> MGSSHHHHHSSGENLYFQGHMGKYTKKFNEVRSTDRPLVGGKCASLGEMVQAGLPVPDGFAVTIDAYEDFRDDSDLRAELRSLVFGVDPDSSKSLQDAHDQAVALVLGRNLPAAIEDEIREAYLTLSRETARRRGTGDTDRIPVAVRSSSVDEDGDAASFAGQQETYLWVVGADDVIAKVRECWASLYTPQAIAYRAGMSETDAAEASKISVAVQLMADADVAGVMFTVSPRTGDRSVIAINASWGLGQSVVSGEVTPDEYWLSKIGPTLTSSRIASKEHEYVPAPDGTGVIFREVEQARREVSCLSDSELMQLAEIGLRV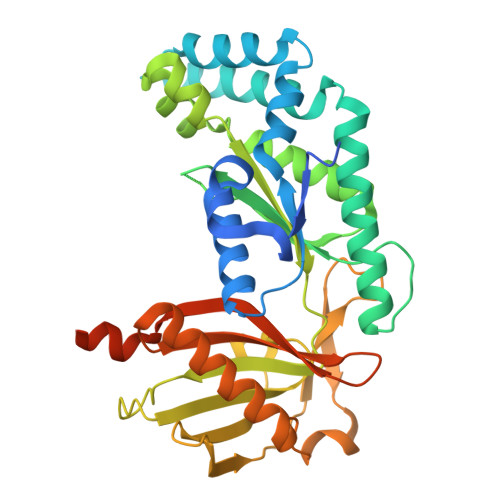EEHYGCPQDIEWALEHDSDGTSRVMLLQSRPETNWKKRKEEKSKRTSSATSNLLGFVSAAAKGQTR UdgX excises uracil from uracil-containing DNA to concurrently form a covalent bond with the resulting AP-DNA. Structurally, UdgX is highly similar to family-4 UDGs (F4-UDGs). However, UdgX is unique in possessing a flexible R-loop (105KRRIH109). Our earlier studies allowed us to propose a reaction mechanism of UdgX, which involves the formation of a covalent bond between H109 of UdgX with the C1′ position of the target deoxyribose sugar concurrently with the uracil excision from this site in DNA.

To evaluate this in more detail, we generated a Q53A mutant wherein the motif A of MsmUdgX was changed to GEAPG to correspond to the motif A of family 4 UDGs. Subsequently, we incorporated the Q53A mutation with the H109S mutant to investigate its role in a surrogate assay of uracil excision (with turnover). The Q53A mutation in the H109S mutant increased its uracil excision activity. Further, the kinetic parameters of uracil excision showed an increase of >2-fold in the Kcat/Km of the double mutant. When compared with the structure of UdgX (wild type), the hydrogen bonding interactions observed between Q53 with N of K97 and O of K110 were lost in H109S/Q53A double mutant due to the absence of Gln side chain in the mutant. This would likely change the positioning of the R-Loop near the active site, leading to an increase in the activity of the H109S/Q53A double mutant, compared to the H109S single mutation. Taken together, these observations suggest that the evolution of Q53 in UdgX (from A53/G53 in family 4 UDGs) disfavours uracil excision activity. Further, as shown by the uracil excision activity of the H109S/Q53A double mutant, the evolution of Q53 (from A or G in family 4 UDGs), appears also to dampen the uracil excision activity. The Q53A mutant supports that UdgX specific evolution of Q53 occurred essentially to stabilize the R-loop conformation.

> AGAQDFVPHTADLAELAAAAGECRGCGLYRDATQAVFGAGGRSARIMMIGEAPGDKEDLAGLPFVGPAGRLLDRALEAADIDRDALYVTNAVKHFKFTRAAGGKRRISKTPSRTEVVACRPWLIAEMTSVEPDVVVLLGATAAKALLGNDFRVTQHRGEVLHVDDVPGDPALVATVHPSSLLRGPKEERESAFAGLVDDLRVAADV> MGWSLPKEKGLILCLWNKFCRWFHRRESWAQSRDEQNLLQQKRIWESPLLLAAKENNVQALYKLLKFEGCEVHQKGAMGETALHIAALYDNNEAAQVLMEAAPELVFEPMTSELYEGQTALHIAVINQNVNLVRALLARGASVSARATGSVFHYRPHNLIYYGEHPLSFAACVGSEEIVRLLIEHGADIRAQDSLGNTVLHILILQPNKTFACQMYNLLLSYDGGDHLKSLELVPNNQGLTPFKLAGVEGNIVMFQHLMQKRKHIQWTYGPLTSTLYDLTEIDSSGDDQSLLELIVTTKKREARQILDQTPVKELVSLKWKRYGRPYFCVLGAIYVLYIICFTMCCVYRPLKPRITNRTNPRDNTLLQQKLLQEAYVTPKDDLRLVGELVSIVGAVIILLVEIPDIFRLGVTRFFGQTILGGPFHVIIVTYAFMVLVTMVMRLTNSDGEVVPMSFAL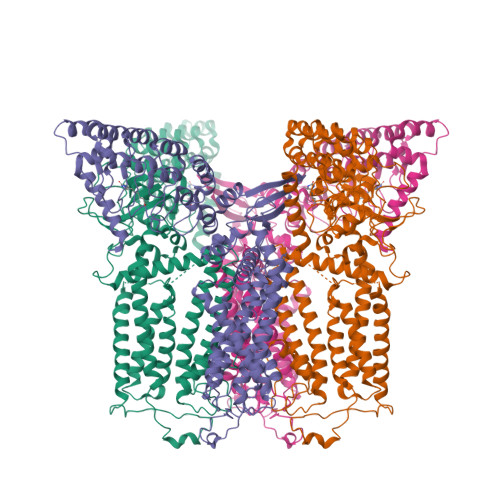VLGWCNVMYFARGFQMLGPFTIMIQKMIFGDLMRFCWQMAVVILGFASAFYIIFQTEDPDELGHFYDYPMALFSTFELFLTIIDGPANYDVDLPFMYSITYAAFAIIATLLMLNLLIAMMGDTHWRVAHERDELWRAQVVATTVMLERKLPRCLWPRSGICGREYGLGDRWFLRVEDRQDLNRQRIRRYAQAFQQQDDLYSEDLEKDSGEKLVPR> MKADNPFDLLLPAAMAKVAEEAGVYKATKHPLKTFYLAITAGVFISIAFVFYITATTGTGTMPFGMAKLVGGICFSLGLILCVVCGADLFTSTVLIVVAKASGRITWGQLAKNWLNVYFGNLVGALLFVLLMWLSGEYMTANGQWGLNVLQTADHKVHHTFIEAVCLGILANLMVCLAVWMSYSGRSLMDKAFIMVLPVAMFVASGFENSIANMFMIPMGIVIRDFASPEFWTAVGSAPE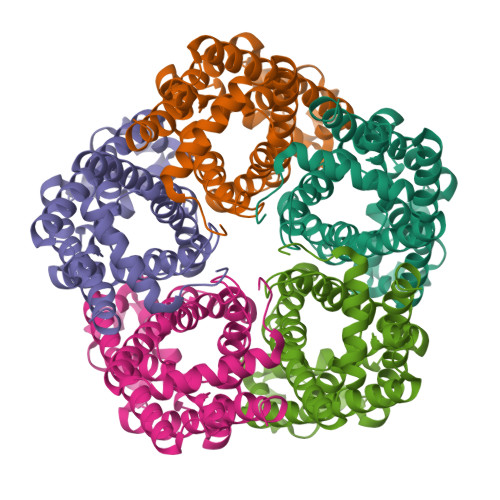NFSHLTVMNFITDNLIPVTIGNIIGGGLLVGLTYWVIYLRENDHH> MDPIGINKVLDHLAPSELIKPVKSCHNKPSVLVLDDRIVDAATKDLYVNGFQEEIQYQNPTPENLQHMFHQGIEILDSARMINVTHLALWKPSSFKLGNPVDFALDDNYDTFWQSDGGQPHQLDIMFSKRMDICVMAIFFSMIADESYAPSLVKVYAGHSPSDARFYKMLEVRNVNGWVALRFLDNREDDQLLKCQFIRLLFPVNHENGKDTHLRGIRLYVPSNEPHQDTHEWAQTLPETNNVFQDAILR;> MSTNLNPFMNNTPSSSPLKGSESKRVSKRPISSSSSASLLSSPSRRSRPSTVYGDRYIPSRTDIDFNSIVSISSMASVPALNPSSTEDQVEYQKERQAHETYNTLLKNELFGEMLSKDTVGSESSIDRIKNTRPSTRGNVHAENTTRHGYELERVSTPPPEAAGLEEFSPHSTPVTPRRLFTSQQDEITRPSSNSVRGASLLTYQQRKGRRLSAASLLQSQFFDSMSPVRPDSKQLLLSPGKQFRQIAKVPYRVLDAPSLADDFYYSLIDWSSTDVLAVALGKSIFLTDNNTGDVVHLCDTENEYTSLSWIGAGSHLAVGQANGLVEIYDVMKRKCIRTLSGHIDRVACLSWNNHVLTSGSRDHRILHRDVRMPDPFFETIESHTQEVCGLKWNVADNKLASGGNDNVVHVYEGTSKSPILTFDEHKAAVKAMAWSPHKRGVLATGGGTADRRLKIWNVNTSIKMSDIDSGSQICNMVWSKNTNELVTSHGYSKYNLTLWDCNSMDPIAILKGHSFRVLHLTLSNDGTTVVSGAGDETLRYWKLFDKPKAKVQPNSLIFDAFNQIR;> MTSKPSTRNDYLPRETHNGEYTGDSPEWQLQINITNKIGGINGDIWLSRDGRSVKWCIEDQCLRQFTYNQKIIKAGYIDFEKTPDCFVVVLSDIAHVYMLKNGGSTTVCFPFQIGNAFWYANGVILERETSASFMDGGYDLKPIEFDLKHKYITLTDPMAPFGLISITNTFKGGINSASGNKTDILQDFQLVLFPSDKDKCIAVFLDRNSKVLRFYYSRILSSDQSRKGELTISSTKKTGLDAAGNSQKSGGISKDLRKFSHLTRRSTSINSNSHDFNAAERVLSGNVGNASGRTDIFALPSSCSRRSLSATLDRMGNNIAPTNRAAPSGFFDSSSANTATHSNITPVSQPMQQQQQEYLNQTATSSKDIVLTEISSLKLPDDIIFTSRRLSSILSKLKFLSLRFERREGLLIFHEPTHFCKIWLIDLLPDVLDSIPFKIYGNSPQNMIRLENLKLKEPSRIQAMYIHELLESCLILVSEGQNKEEYKACLYDPFVKITSPSKNISEELTKQNSLPSLQKLFPYPETSFTKLCFEAVKYITSPAFNISFIFLWQSAYSILLSRANDDVVGGLKMEHDAFSLVLSLLILPIPSSSAQEYQEYKEIYERDLFQHLKQDSEITSSVLPRIVIGLHLIREEYSLNVLCRNEHALLGQFLRFATAAMGWPDLWQSYYVPKMDSESKTFLHPREQNSTFFHPLDEPPSITKSLYSITENSSIPLCPFISFSRLVATDTQVELRITPRSFKILGLYELVHSPNFLPDYVLGILSSFKVDKDELQTYPLGILVPLQNILKILEDKLSEVRDNLELLDRADLQRCSAIINSIRSDSKEVLKRGQRDSYMLCKVPLAKNRSSLSKKPSDIYSILSEIVKSASQVPLDGSAMRMSNIQDDEDIDEGRSLKLNAGLIFSEDKRFTHVVSLLAYYRPTKTQFFTTKTEYAQILAQKKYFAKIMALRTCTNGVGWGAVAYATEKPISTQKWVIQPLNLISVFPDDTKITVKAPEDIAHDIVEWGQFHAGVSSGLRISKKATGITGSWIAFNKPKELDAYHGGFLLGLGLNGHLKNLEEWHIYNYLSPRNTHISIGLLLGMSSSMKGSMDSKLIKVISVHLVAFLPSGSSDLNIDLKLQTAGIIGMGMLYLNSRHKRMSDSIFAQLVSLLNVNDEMVADEEYRLAAGISLGLINLGAGQTKLRKWDSSLLGLGDDLPEDVYDSSDVEQNVMYEDLTTKLLEIVTSTYDVENDWIPENSQIGAVIAIMFLFLKSNNFGISNMLKVDLKEILKANINTRPELLMYREWASNMILWEFIGDDLSFIMKDVDIGVKFSELNTDLLPIYYTMAGRILAMGIRFASTGNLKIRNILLSLVDKFLPLYQYPGKQNLDFRLTISVINVLTNVIVVSLSMVMCASGDLEVLRRVKYLHEVASGPYSDLFQEIPSSKSDVSGVTQVTSNTNTPGNSDRERVDETAASLDDERSSNGSDISDPTAYLEDKKDIDDHYGKFISTNLALGFLFLGSGQYALNTSTLESIAFLSMSVLPTYTTPHPLQELKHFWSMAVEPRCLVIKDISTGDAVNNVPIELVVEEDVEKEEVIREISTPCLLPDFSKIKSIRVKMHGYFPLEVNFTKDYSASDFFSGGTIIYIQRKSESVFENKASFRNVEDIHVA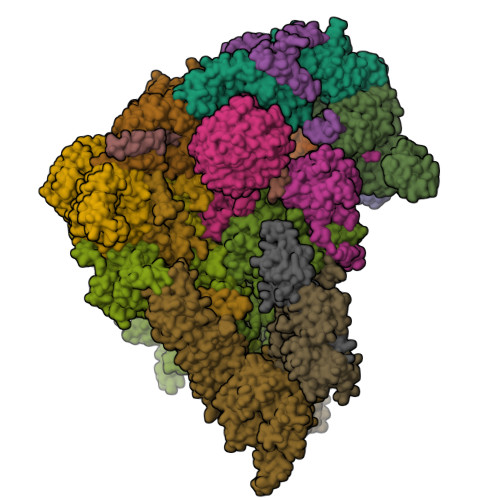LKRKAAESKNYSRLNLKNEQGNTTSSQLVESLGIQDLTMVELDTLLSAGNNTALTDSESYNLGLLCSDKNSGDILDCQLELWYKSFGPHDE;>MNDDSQDKIIHDIRIQLRKAATELSRWKLYGSSKWAAEALAGLAEAIDVDQTHSLADESPLRNKQGVPKQMFEIPQNGFGLSETEYDLYLLGSTLFDAKEFDRCVFFLKDVTNPYLKFLKLYSKFLSWDKKSQESMENILTTGKFTDEMYRANKDGDGSGNEDINQSGHQRANLKMVSNEHESQSNISSILKEINTFLESYEIKIDDDEADLGLALLYYLRGVILKQEKNISKAMSSFLKSLSCYSFNWSCWLELMDCLQKVDDALLLNNYLYQNFQFKFSENLGSQRTIEFNIMIKFFKLKVFEELNGQLEDYFEDLEFLLQVFPNFTFLKAYNATISYNNLDYVTAESRFDDIVKQDPYRLNDLETYSNILYVMQKNSKLAYLAQFVSQIDRFRPETCCIIANYYSARQEHEKSIMYFRRALTLDKKTTNAWTLMGHEFVELSNSHAAIECYRRAVDICPRDFKAWFGLGQAYALLDMHLYSLYYFQKACTLKPWDRRIWQVLGECYSKTGNKVEAIKCYKRSIKASQTVDQNTSIYYRLAQLYEELEDLQECKKFMMKCVDVEELLEGIVTDETVKARLWLAIFEIKAGNYQLAYDYAMGVSSGTSQEIEEARMLARECRRHM[2x];> MNQNGDKNEGKLFQLPSLPPWKTPRFNKANFNNFTTPLRKRSTRVINDDSMPITGEVLEERTADDLYGINMDVDEVDYLNTLSHIEEEKQYDYSPFCERNTLRESRIDSFLKAERAAHCLVFHKVGHLDGIDSYRPDIDIMCGEEANKYDSANPEGNGSMLLESVPGCNKEDLERLSRREFVTNSKPNMRRLDDIINHETNALKSFWNDSGLVNSLQSHHLHEEYLLLQEELKNVYKIKCHDRVPIESLRDKCRRHYSNEDSSFL;>MAVNPELAPFTLSRGIPSFDDQALSTIIQLQDCIQQAIQQLNYSTAEFLAELLYAECSILDKSSVYWSDAVYLYALSLFLNKSYHTAFQISKEFKEYHLGIAYIFGRCALQLSQGVNEAILTLLSIINVFSSNSSNTRINMVLNSNLVHIPDLATLNCLLGNLYMKLDHSKEGAFYHSEALAINPYLWESYEAICKMRATVDLKRVFFDIAGKKSNSHNNNAASSFPSTSLSHFEPRSQPSLYSKTNKNGNNNINNNVNTLFQSSNSPPSTSASSFSSIQHFSRSQQQQANTSIRTCQNKNTQTPKNPAINSKTSSALPNNISMNLVSPSSKQPTISSLAKVYNRNKLLTTPPSKLLNNDRNHQNNNNNNNNNNNNNNNNNNNNNNNNIINKTTFKTPRNLYSSTGRLTTSKKNPRSLIISNSILTSDYSITLPEIMYNFALILRSSSQYNSFKAIRLFESQIPSHIKDTMPWCLVQLGKLHFEIINYDMSLKYFNRLKDLQPARVKDMEIFSTLLWHLHDKVKSSNLANGLMDTMPNKPETWCCIGNLLSLQKDHDAAIKAFEKATQLDPNFAYAYTLQGHEHSSNDSSDSAKTCYRKALACDPQHYNAYYGLGTSAMKLGQYEEALLYFEKARSINPVNVVLICCCGGSLEKLGYKEKALQYYELACHLQPTSSLSKYKMGQLLYSMTRYNVALQTFEELVKLVPDDATAHYLLGQTYRIVGRKKDAIKELTVAMNLDPKGNQVIIDELQKCHMQE[2x];>[2x]MIRRAPTTLQLSHDDVTSLIDDLNEQKLKQQLNIEKTKYFQGKNGGSLHSNTDFQDTSQNIEDNNNDNDNDIDEDDDMSSYNDKAASVAHTRVLNSLHLSTDSNTAHETSNANDNHNPFYIREE;> MSSSSYRDSYFQYRHLPAPHHILYAEWNQDILALPDEVANITMAMKDNTRTDAEEGRAPQDGERNSNVRESAQGKALMTSEQNSNRYWNSFHDEDDWNLFNGMELESNGVVTFAGQAFDHSLNGGTNSRNDGANEPRKETITGSIFDRRITQLAYARNNGWHELALPQSR;>[2x]MKFCLYCCHCYIVICGKATHYYKSSKATSNLKSSNRVLMRNPMSPSEQHSQHNSTLAASPFVSNVSAARTQQSLPTDAQNDRLQQPWNRTNTATSPYQSLANSPLIQKLQANIMTPHQPSANSNSNSNSITGNVVNDNNLLASMSKNSMFGSTIPSTLRKVSLQREYKDSVDGVVRDEDNDEDVHNNGDAAANANNDRESKLGHNGPLTTTTLTTTTTATQLDVSELSAIERLRLWRFDALMQHMYRTAEYIADKVYNISNDPDDAFWLGQVYYNNNQYVRAVELITRNNLDGVNILCRYLLGLSFVKLQRFDDALDVIGEYNPFSEDPSTTAANTMSNNGNNSNTSQPVTDGGIKMESSLCFLRGKIYFAQNNFNKARDAFREAILVDIKNFEAFEMLLSKNLLTPQEEWDLFDSLDFKEFGEDKEIMKNLYKINLSKYINTEDITKSNEILAKDYKLADNVDVVRSKVDICYTQCKFNECLELCETVLENDEFNTNILPAYIGCLYELSNKNKLFLLSHRLAETFPKSAITWFSVATYYMSLDRISEAQKYYSKSSILDPSFAAAWLGFAHTYALEGEQDQALTAYSTASRFFPGMHLPKLFLGMQFMAMNSLNLAESYFVLAYDICPNDPLVLNEMGVMYFKKNEFVKAKKYLKKALEVVKDLDPSSRTTISIQLNLGHTYRKLNENEIAIKCFRCVLEKNDKNSEIHCSLGYLYLKTKKLQKAIDHLHKSLYLKPNNSSATALLKNALELNVTLSLDASHPLIDKSNLMSQASKDKASLNKKRSSLTYDPVNMAKRLRTQKEIFDQNNKALRKGGHDSKTGSNNADDDFDADMELEKSSIPENLYF;> MARALRDISLFNDIRKDQNSAGAKHERYNMRDLRSKKNQHVNGIDDYEDDSLDRFIRRKKSRVVKYIPSLSAYNVFNEFPYYPTSASQLLDGKLDEFLMLSEQYKSRLPKIRKLGWNRFKPIGINKTMYELEMLRSRARAQNAEGNNEEDFRQHDSREEDPRNNGSIGRVILPHILQENEEYDTGEGVTGLHSMPNDSMAILANNSANNSQNEEVSEEDEISYDYDAEFDHVVDEDDNEEGEVPGEGVEGIEVQRERIVPDDLLMRPTSLSRSLQQFVEEAHHLDRNPYDIDSDNDGEDSKVELDMNPDFEDDVGREHDYNSEYSQEPTSYGGITPDLASNWRNWTRERITSLDELMERRARQQRGQD;> MSKYGPLGITNFITPYDLCILILIHAHCSQDNGISVPTAVFLRLISPTRPSLEWNPLLKDNSNLRSSSIVPPPVLPILDNIIRILLDDKDGNKIALTLMGYLEAINGLDSINRLMMDLEKNCLVNNYRSMKMRTTSTRRQMTRASFLGTFLSTCIRKYQIGDFEMRETIWINLQNFKTVFKHTPLWLRFKDNVHIQKVKNCLLANDEISVEDQQMVEFFQHFNNGNDADSKTMNEENYGTLISIQHLQSIVNRQIVNWLDNTEFNLMGQEETSSTYEEQSGLVFDLLDTLSLNDATKFPLIFILKYLEAIKENSYQTALDSLHNYFDYKSTGNSQNYFHISLLSLATFHSSFNECDAAINSFEEATRIARENKDMETLNLIMIWIINFIEVHPEYANRFYITVEQIIKYLKNSSDVEDANIFSNAYKFETLLSMVKESKTAEVSSSLLKFMAITLQNVPSQNFDLFQSLVSYEVKFWKELGYESISDVYEKFLSKTSSSSLRNYDSSIINQDIKVAFKALEEDDFLKVKQYLLKSESLELDYDQKINLKYLRVKYLVKIGDYDLSMRLINQYVKECCEEVADSNWRFKFEIESINVLLLSDVGIRSLPKIIKLIDEYKEIGNPLRCVILLLKLCEVLIQVGKSMEAECLISCNLSTILEFPFVRKKTDELLESLSVEEDRDVQMT;> MSSPINDYFIDYNPLFPIFATRIAKGLAIYRVSDHARLAVIPIRNINLVANYDWDTTTGKFLSIFFKDGTIRIHDIFKDGRLVSFLRIPSTKISKGIWDRIPLRYEPNNRDFACNIIDDLPKLIRFVKDSKRINIVPYTQPNSLWRGPDEDDLDSNEKLDVHVVFNEGNDKITVFFNGDYAVFLSVDNIENENSLKSIIKVQDGFYQCFYEDGTVQTLNLGPLLQSKSSVNLLNYIMVIKELIGYMLTHLEFINRELATPYLDFVKRLCDEAYGYGKLKSELEALFLLGEISCDLEDWLCNSVGEKNFKRWKYLGCEAYQKTVQILTLIFVPACERIIIYVEKLRAILQAFSIQNKLSYTSDLTAVEVLLKSSQKLLTMTLNSIIGLGRDETLFEKFFIWFNDRLHEALDEDYKLKFQFEDDLYFGYDLLSYFDRILSKKGTEPSSIIDVKLYRDLINSMSDMEKDIAQSNVNSHIQQHILVDLKTDVFAQKYPSSQINLLDAIKLPKHNYIVYLIQVTKHNSAQEPFSEENKKKLYIGTLKDENLGIISKESSVKIPALFKSYRLSSTRFVPNRVHSLLRDIGLSDSNYHSSHVTDYRGENYENEEDDGTIAIPAYIRENRENDDFIACTAKVSVDGRSASLVFPKEKQNV;> MTGHVSKTSHVPKGRPSSLAKKAAKRAMAKVNSNPKRASGHLERVVQSVNDATKRLSQPDSTVSVATKSSKRKSRDTVGPWKLGKTLGKGSSGRVRLAKNMETGQLAAIKIVPKKKAFVHCSNNGTVPNSYSSSMVTSNVSSPSIASREHSNHSQTNPYGIEREIVIMKLISHTNVMALFEVWENKSELYLVLEYVDGGELFDYLVSKGKLPEREAIHYFKQIVEGVSYCHSFNICHRDLKPENLLLDKKNRRIKIADFGMAALELPNKLLKTSCGSPHYASPEIVMGRPYHGGPSDVWSCGIVLFALLTGHLPFNDDNIKKLLLKVQSGKYQMPSNLSSEARDLISKILVIDPEKRITTQEILKHPLIKKYDDLPVNKVLRKMRKDNMARGKSNSDLHLLNNVSPSIVTLHSKGEIDESILRSLQILWHGVSRELITAKLLQKPMSEEKLFYSLLLQYKQRHSISLSSSSENKKSATESSVNEPRIEYASKTANNTGLRSENNDVKTLHSLEIHSEDTSTVNQNNAITGVNTEINAPVLAQKSQFSINTLSQPESDKAEAEAVTLPPAIPIFNASSSRIFRNSYTSISSRSRRSLRLSNSRLSLSASTSRETVHDNEMPLPQLPKSPSRYSLSRRAIHASPSTKSIHKSLSRKNIAATVAARRTLQNSASKRSLYSLQSISKRSLNLNDLLVFDDPLPSKKPASENVNKSEPHSLESDSDFEILCDQILFGNALDRILEEEEDNEKERDTQRQRQNDTKSSADTFTISGVSTNKENEGPEYPTKIEKNQFNMSYKPSENMSGLSSFPIFEKENTLSSSYLEEQKPKRAALSDITNSFNKMNKQEGMRIEKKIQREQLQKKNDRPSPLKPIQHQELRVNSLPNDQGKPSLSLDPRRNISQPVNSKVESLLQGLKFKKEPASHWTHERGSLFMSEHVEDEKPVKASDVSIESSYVPLTTVATSSRDPSVLAESSTIQKPMLSLPSSFLNTSMTFKNLSQILADDGDDKHLSVPQNQSRSVAMSHPLRKQSAKISLTPRSNLNANLSVKRNQGSPGSYLSNDLDGISDMTFAMEIPTNTFTAQAIQLMNNDTDNNKINTSPKASSFTKEKVIKSAAYISKEKEPDNSDTNYIPDYTIPNTYDEKAINIFEDAPSDEGSLNTSSSESDSRASVHRKAVSIDTMATTNVLTPATNVRVSLYWNNNSSGIPRETTEEILSKLRLSPENPSNTHMQKRFSSTRGSRDSNALGISQSLQSMFKDLEEDQDGHTSQADILESSMSYSKRRPSEESVNPKQRVTMLFDEEEEESKKVGGGKIKEEHTKLDNKISEESSQLVLPVVEKKENANNTENNYSKIPKPSTIKVTKDTAMESNTQTHTKKPILKSVQNVEVEEAPSSDKKNWFVKLFQNFSSHNNATKASKNHVTNISFDDAHMLTLNEFNKNSIDYQLKNLDHKFGRKVVEYDCKFVKGNFKFKIKITSTPNASTVITVKKRSKHSNTSSNKAFEKFNDDVERVIRNAGRS;> MSFQITPTRDLKVITDELQTLSSYIFHTNIVDDLNSLLTWMSPNDAKSNHQLRPPSLRIKNIIKVLFPNNATTSPYSMINTSQANNSIVNEGNTNKELQLQLFSTLKEFYIFQVRYHFFLHFNNINYLKDIQRWENYYEFPLRYVPIFDVNVNDWALELNSLRHYLLNRNIKFKNNLRTRLDKLIMDDDFDLADNLIQWLKSANGSLSSTELIVNALYSKINKFCEDNMSRVWNKRFMIMETFNKFINQYWSQFSKLVGCPEDDHELTTTVFNCFESNFLRIRTNEIFDICVLAYPDSKVTLLELRKIMKDFKDYTNIVTTFLSDFKKYILNPSVTTVDALLRYVKTIKAFLVLDPTGRCLHSITTFVKPYFQERKHLVNVLLYAMLDLPEEELKEKINFNVDMKALLSLVDTLHDSDINQDTNITKRDKNKKSPFLWNLKVKGKRELNKDLPIRHAMLYEHILNYYIAWVPEPNDMIPGNIKSSYIKTNLFEVLLDLFESREFFISEFRNLLTDRLFTLKFYTLDEKWTRCLKLIREKIVKFTETSHSNYITNGILGLLETTAPAADADQSNLNSIDVMLWDIKCSEELCRKMHEVAGLDPIIFPKFISLLYWKYNCDTQGSNDLAFHLPIDLERELQKYSDIYSQLKPGRKLQLCKDKGKVEIQLAFKDGRKLVLDVSLEQCSVINQFDSPNDEPICLSLEQLSESLNIAPPRLTHLLDFWIQKGVLLKENGTYSVIEHSEMDFDQAQKTAPMEIENSNYELHNDSEIERKYELTLQRSLPFIEGMLTNLGAMKLHKIHSFLKITVPKDWGYNRITLQQLEGYLNTLADEGRLKYIANGSYEIVKNGHKNS;> MKVKINEVHSVFAWSWHIPSTSDEDAANNDPIGNDEDEDVCGICRASYNGTCPSCKFPGDQCPLVIGLCHHNFHDHCIYRWLDTPTSKGLCPMCRQTFQLQKGLAINDAHVQKFVEIVSRRREEMIEEGVAEEFVDFDEPIRQNTDNPIGRQQVDTILDEDFLLR> MIRLYPEQLRAQLNEGLRAAYLLLGNDPLLLQESQDAVRQVAAAQGFEEHHTFSIDPNTDWNAIFSLCQAMSLFASRQTLLLLLPENGPNA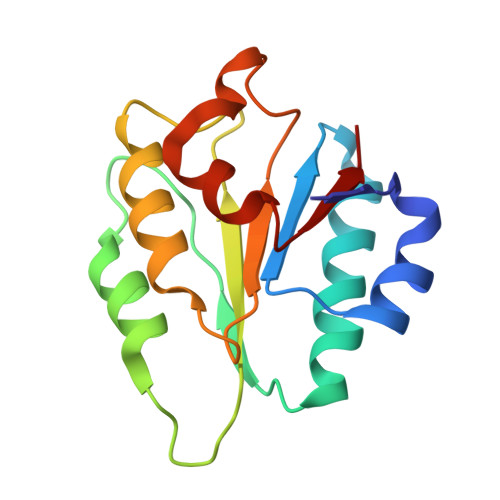AINEQLLTLTGLLHDDLLLIVRGNKLSKAQENAAWFTALANRSVQVTCQ>MPAIRKARGWVPPGYNYLGPFNQDFNKKPTNPSDNAARKHDLEYNKLIKQGHNPYWNYNHADEDFIKETDQATDWGGKFGNFVFRAKRALAPELAPPAKKKTKTKHTEPEYSHKHIKAGTKRGKPFYLFVNLARKKARMTDTQDVSEQQSDQPSVASTNAKAGGGGGGGGSGVGHSTGNYNNRTEFYYHGDEVTIVCHSSRHIHLNMSESEEYKIYDTDRGPRFPTDQTLQGRDTINDSYHAQVETPWFLINPNSWGTWMNPADFQQLTTTCREVTLEHLDQTLDNIVIKTVSKQGSGAEETTQYNNDLTALLQVALDKSNQLPWVADNMYLDSLGYIPWRPCKLKQYSYHVNFWNTIDIISGPQQNQWQQVKKEIRWDDLQFTPIETTTEIDLLRTGDSWTSGPYKFNTKPTQLSYHWQSTRHTGSVHPTDPPNAIGQQGQNIRDINGWQWGDRSDPMSAATRVSNFHIGYSWPEWRIHYGSGGPAINPGAPFSQAPWSTDPQVRLTQGASEKAIFDYNHGDDDPAHRDQWWQNNLPITGQTNWAPKNAHQANLSSNVPSRQEFWTQDYHNTFGPFTAVDDVGIQYPWGAIWTKTPDTTHKPMMSAHAPFICKDGPPGQLLVKLAPNYTENLQTDGLGNNRIVTYATFWWTGKLILKGKLRLPRQF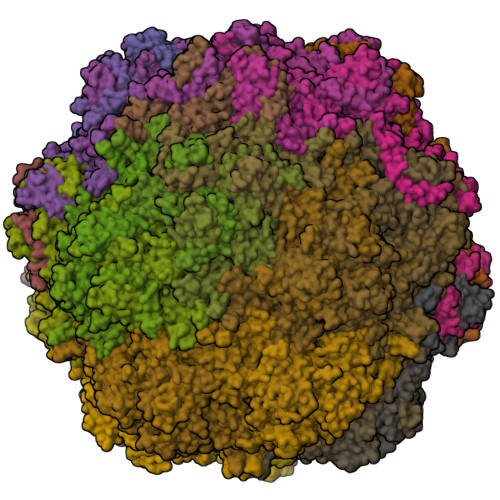NLYNLPGRPRGTEAKKFLPNEIGHFELPFMPGRCMPNYTM[60x]> AVKNCSHLECFYNSRANVSCMWSHEEALNVTTCHVHAKSNLRHWNKTCELTLVRQASW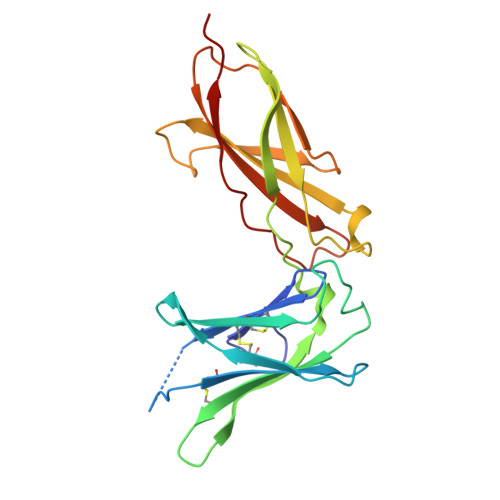ACNLILGSFPESQSLTSVDLLDINVVCWEEKGWRRVKTCDFHPFDNLRLVAPHSLQVLHIDTQRCNISWKVSQVSHYIEPYLEFEARRRLLGHSWEDASVLSLKQRQQWLFLEMLIPSTSYEVQVRVKAQRNNTGTWSPWSQPLTFRTRPA>[2x]GSRKIIHVDMDCFFAAVEMRDNPALRDIPIAIGGSRERRGVISTANYPARKFGVRSAMPTGMALALCPHLTLLPGRFDAYKE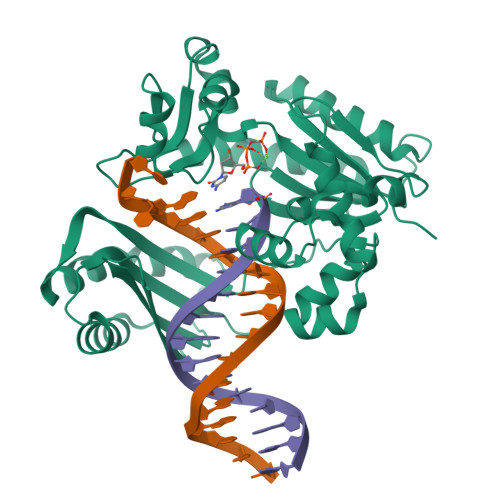ASNHIREIFSRYTSRIEPLSLDEAYLDVTDSVHCHGSATLIAQEIRQTIFNELQLTASAGVAPVKFLAKIASDMNKPNGQFVITPAEVPAFLQTLPLAKIPGVGKVSAAKLEAMGLRTCGDVQACDLVMLLKRFGKFGRILWERSQGIDERDVNSERLRKSVGVERTMAEDIHHWSECEAIIERLYPELERRLAKVKPDLLIARQGVKLKFDDFQQTTQEHVWPRLNKADLIATARKTWDERRGGRGVRLVGLHVTLLDP>TNLVAEPFAKLEQDFGGSI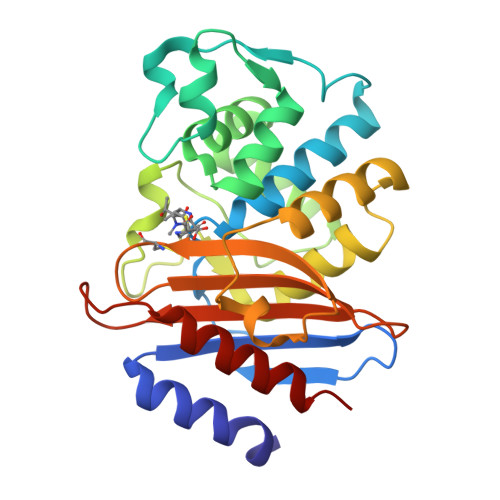GVYAMDTGSGATVSYRAEERFPLCGSFKGFLAAAVLARSQQQAGLLDTPIRYGKNALVPWSPISEKYLTTGMTVAELSAAAVQYSDNAAANLLLKELGGPAGLTAFMRSIGDTTFRLDRWELELNSAIPGDARDTSSPRAVTESLQKLTLGSALAAPQRQQFVDWLKGNPTGNHRIRAAVPADWAVGDKTGTCGVYGTANDYAVVWPTGRAPIVLAVYTRAPNKDDKHSEAVIAAAARLALEGLG[2x]> GPGSCPTHADSLNNLANIKREQGNIEEAVRLYRKALEVFPEFAAAHSNLASV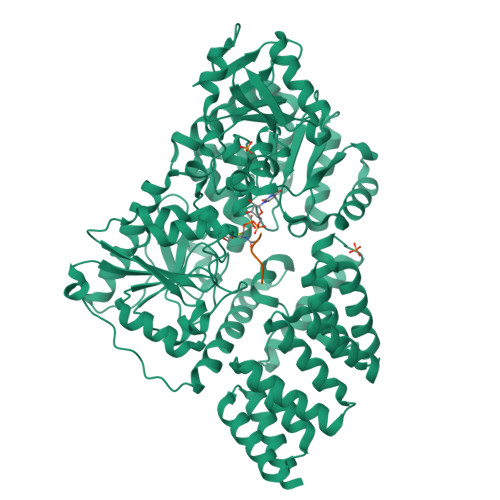LQQQGKLQEALMHYKEAIRISPTFADAYSNMGNTLKEMQDVQGALQCYTRAIQINPAFADAHSNLASIHKDSGNIPEAIASYRTALKLKPDFPDAYCNLAHCLQIVCDWTDYDERMKKLVSIVADQLEKNRLPSVHPHHSMLYPLSHGFRKAIAERHGNLCLDKINVLHKPPYEHPKDLKLSDGRLRVGYVSSDFGKHPTSHLMQSIPGMHNPDKFEVFCYALSPDDGTNFRVKVMAEANHFIDLSQIPCNGKAADRIHQDGIHILVNMNGYTKGARNELFALRPAPIQAMWLGYPGTSGALFMDYIITDQETSPAEVAEQYSEKLAYMPHTFFIGDHANMFPHLKKKAVIDFKSNGHIYDNRIVLNGIDLKAFLDSLPDVKIVKMKCPDGGDNADSSNTALNMPVIPMNTIAEAVIEMINRGQIQITINGFSISNGLATTQINNKAATGEEVPRTIIVTTRSQYGLPEDAIVYCNFNQLYKIDPSTLQMWANILKRVPNSVLWLLRFPAVGEPNIQQYAQNMGLPQNRIIFSPVAPKEEHVRRGQLADVCLDTPLCNGHTTGMDVLWAGTPMVTMPGETLASRVAASQLTCLGCLELIAKNRQEYEDIAVKLGTDLEYLKKVRGKVWKQRISSPLFNTKQYTMELERLYLQMWEHYAAGNKPDHMIKPVE;> KKVAVSRAA>[8x]SETQRQFSRYFIEFEELQLLGKGAFGAVIKVQNKLDGCCYAVKRIPINPASRQFRRIKGEVTLLSRLHHENIVRYYNAWIERHERPSVTTEAVHYLYIQMEYCEKSTLRDTIDQGLYRDTVRLWRLFREILDGLAYIHEKGMIHRNLKPVNIFLDSDDHVKIGDFGLATDHLAFSADSKQDDQTGDLI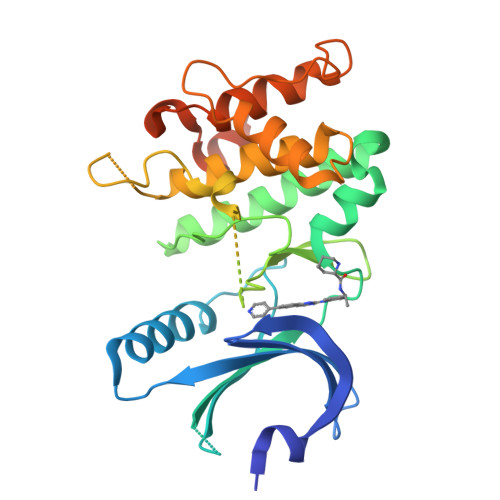KSDPSGHLTGMVGTALYVSPEVQGSTKSAYNQKVDLFSLGIIFFEMSYHPMVTASERIFVLNQLRDPTSPKFPEDFDDGEHAKQKSVISWLLNHDPAKRPTATELLKSELLPPPQMEESELHEVLHHTLT>[2x]MGVRFAGVNIAGFDFGCTTDGTCVTSKVYPPLKNFTGSNNYPDGIGQMQHFVNEDGMTIFRLPVGWQYLVNNNLGGNLDSTSISKYDQLVQGCLSLGAYCIVDIHNYARWNGGIIGQGGPTNAQFTSLWSQLASKYASQSRVWFGIMNEPHDVNINTWAATVQEVVTAIRNAGATSQFISLPGNDWQSAGAFISDGSAAALSQVTNPDGSTTNLIFDVHKYLD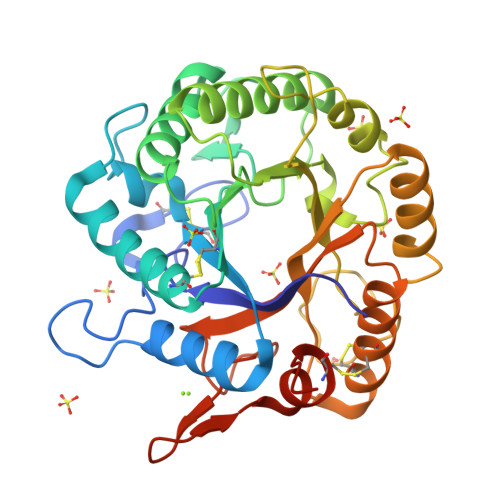SDNSGTHAECTTNNIDGAFSPLATWLRQNNRQAILTETGGGNVQSCIQDMCQQIQYLNQNSDVYLGYVGWGAGSFDSTYVLTETPTSSGNSWTDTSLVSSCLARKGGSGSGHHHHHH>[2x]ARKCSLTGKWTNNLGSIMTIRAVNSRGEFTGTYLTAVAANPGNITLSPLLGIQHKRASQPTFGFTVHWNFSESTTVFTGQ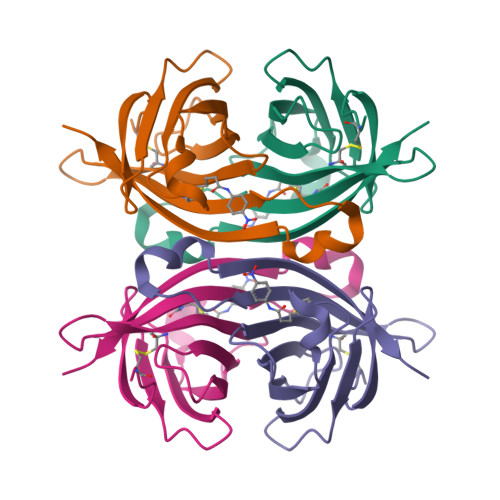CFIDRNGKEVLKTMWLLRSSVNDISYDWKATRVGYNNFTRLSTVEE>HMSTGDFLTKGIELVQKAIDLDTATQYEEAYTAYYNGLDYLMLALKYEKNPKSKDLIRAKFTEYLNRAEQLKKHLESEEANAA[2x];>MNPEKMNNAKVANMPSTEG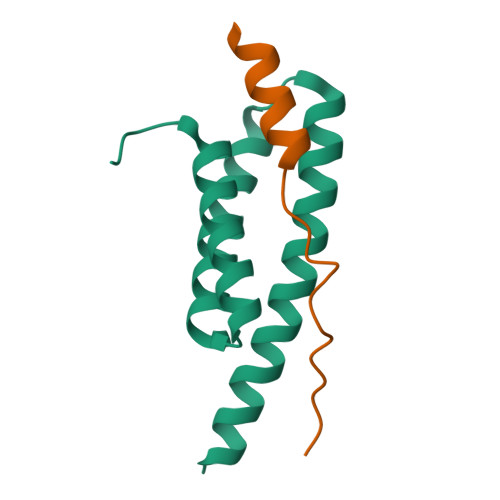LPSLPQGE[2x]> GSPEFIEKNFVISDPRLPDNPIIFASDSFLELTEYSREEILGRNCRFLQGPETDQATVQKIRDAIRDQREITVQLINYTKSGKKFW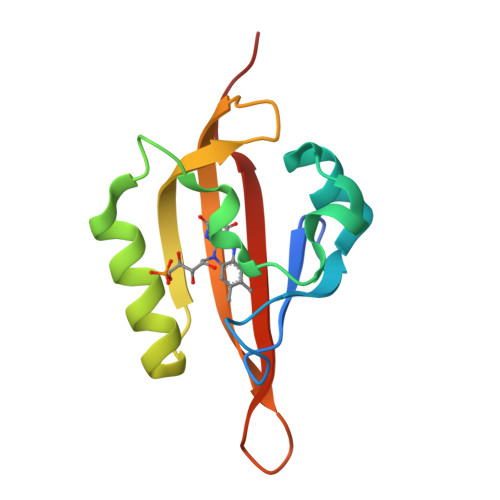NLFHLQPMRDQKGELQYFIGVQLDGSDHV>CTVGPDYRTPDTAAAKIDATASKPYDRSRFESLWWKQFDDPTLNQLVEQSLSGNRDLRVAFARLRAARALRDDVANDRFPVVTSRASADIGKGQQPGVTEDRVNSERYDLGLDSAWELDLFGRIRRQLESSDALSEAAEADLQQLQVSLIAELVDAYGQLRGAQLREKIALSNLENQKESRQLTEQLRDAGVGAELDVLRADARLAATAASVPQLQAEAERARHRIATLLGQRPEELTVDLSPRDLPAITKALPIGDPGELLRRRPDIRAAERRLAASTADVGVATADLFPR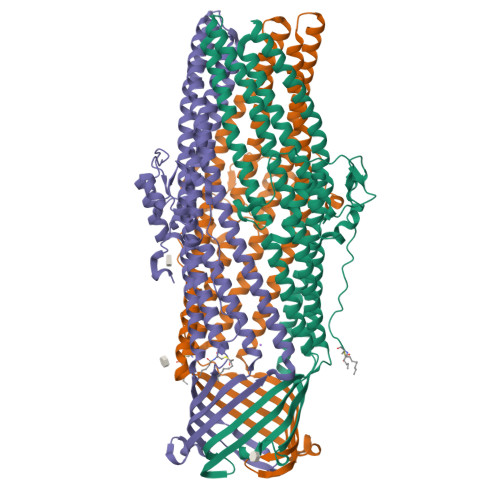VSLSGFLGFTAGRGSQIGSSAARAWSVGPSISWAAFDLGSVRARLRGAKADADAALASYEQQVLLALEESANAFSDYGKRQERLVSLVRQSEASRAAAQQAAIRYREGTTDFLVLLDAEREQLSAEDAQAQAEVELYRGIVAIYRSLGGGWQPSAHHHHHH[3x]>[2x]MVSKNKKLNLKDKYQYLTRDMAWEPTYQDKKDIFPEEDFEGIKITDWSQWEDPFRLTMDAYWKYQAEKEKKLYAIFDAFAQNNGHQNISDARYVNALKLFISGISPLEHAAFQGYSKVGRQFSGAGARVACQMQAIDELRHSQTQQHAMSHYNKHFNGLHDGPHMHDRVWYLSVPKSFFDDARSAGPFEFLTAISFSFEYVLTNLLFVPFMSGAAYN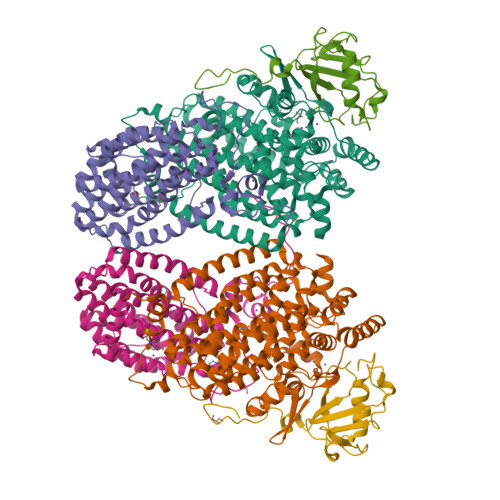GDMATVTFGFSAQSDEARHMTLGLEVIKFILEQHEDNVPIVQRWIDKWFWRGFRLLSLVSMMMDYMLPNKVMSWSEAWEVYYEQNGGALFKDLERYGIRPPKYQDVANDAKHHLSHQLWTTFYQYCQATNFHTWIPEKEEMDWMSEKYPDTFDKYYRPRYEYLAKEAAAGRRFYNNTLPQLCQVCQIPTIFTEKDAPTMLSHRQIEHEGERYHFCSDGCCDIFKHEPEKYIQAWLPVHQIYQGNCEGGDLETVVQKYYHINIGEDNFDYVGSPDQKHWLSIKGRKPADKNQDAA;>[2x]MSIEIKTNSVEPIRHTYGHIARRFGDKPATRYQEASYDIEAKTNFHYRPQWDSEHTLNDPTRTAIRMEDWCAVSDPRQFYYGAYVGNRAKMQESAETSFGFCEKRNLLTRLSEETQKQLLRLLVPLRHVELGANMNNAKIAGDATATTVSQMHIYTGMDRLGIGQYLSRIALMIDGSTGAALDESKAYWMDDEMWQPMRKLVEDTLVVDDWFELTLVQNILIDGMMYPLVYDKMDQWFESQGAEDVSMLTEFMRDWYKESLRWTNAMMKAVAGESETNRELLQKWIDHWEPQAYEALKPLAEASVGIDGLNEARAELSARLKKFELQSRGVSA;>[2x]MSVNALYDYKFEPKDKVENFHGMQLLYVYWPDHLLFCAPFALLVQPGMTFSALVDEILKPATAAHPDSAKADFLNAEWLLNDEPFTPKADASLKEQGIDHKSMLTVTTPGLKGMANAGY> MGKALVIVESPAKAKTINKYLGSDYVVKSSVGHIRDLPTSGSAAKKSADSTSTKTAKKPKKDERGALVNRMGVDPWHNWEAHYEVLPGKEKVVSELKQLAEKADHIYLATNLDREGEAIAWHLREVIGGDDARYSRVVFNEITKNAIRQAFNKPGELNIDRVNAQQARRFMDRVVGYMVSPLLWKKIARGLSAGRVQSVAVRLVVEREREIKAFVPEEFWEVDASTTTPSGEALALQVTHQNDKPFRPVNKEQTQAAVSLLEKARYSVLEREDKPTTSKPGAPFITSTLQQAASTRLGFGVKKTMMMAQRLYEAGYITYMRTDSTNLSQDAVNMVRGYISDNFGKKYLPESPNQYASKENSQEAHEAIRPSDVNVMAESLKDMEADAQKLYQLIWRQFVACQMTPAKYDSTTLTVGAGDFRLKARGRILRFDGWT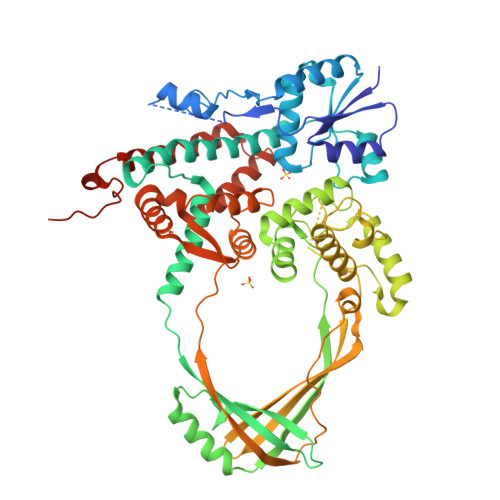KVMPALRKGDEDRILPAVNKGDALTLVELTPAQHFTKPPARFSEASLVKELEKRGIGRPSTYASIISTIQDRGYVRVENRRFYAEKMGEIVTDRLEENFRELMNYDFTAQMENSLDQVANHEAEWKAVLDHFFSDFTQQLDKAEKDPEEGGMRPNQMVLTS> GAHMNDIKQLLWNGELNVLVSIDPSFLMKGSPREIAVLRIRVPRETYLVNYMPLIWNKIKSFLSFDPLTDSEKYFWFEHNKTPIPWNYPVGVLFDCLAGKSATFTTSFENQVKDVLTFLRIHLVMGDSLPPTIIPIASSKTQAEKFWFHQWKQVCFILNGSSKAIMSLSVNEARKFWGSVITRNFQDFIEISNKISSSRPRHIPLIIQTSRTSGTFRISQ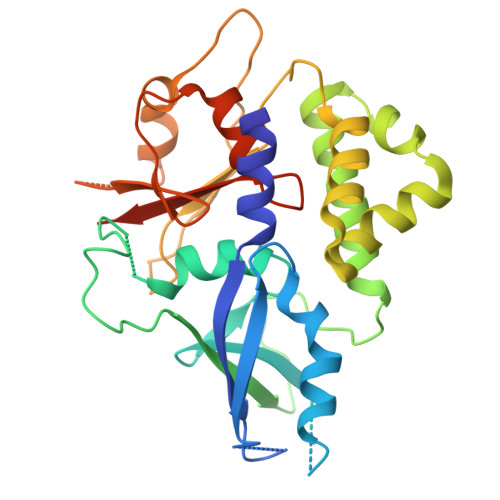PTISMTGVNPTLKDIEGDILDVKEGINGNDVMVICQGIEIPWHMLLYDLYSKLRSFDGFLYITLVPIKGGDKASSEL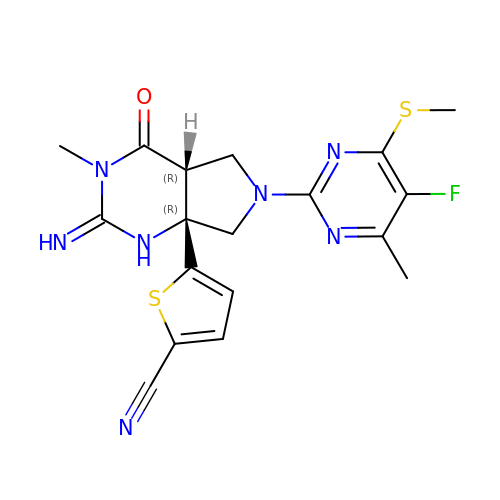5-{(2E,4aR,7aR)-6-[5-fluoro-4-methyl-6-(methylsulfanyl)pyrimidin-2-yl]-2-imino-3-methyl-4-oxooctahydro-7aH-pyrrolo[3,4-d]pyrimidin-7a-yl}thiophene-2-carbonitrile | C18 H18 F N7 O S2 | RVOBSBJZKQOYEK-VOJFVSQTSA-N>[2x]MALVDGFLELERSSGKLEWSAILQKMASDLGFSKILFGLLPKDSQDYENAFIVGNYPAAWREHYDRAGYARVDPTVSHCTQSVLPIFWEPSIYQTRKQHEFFEEASAAGLVYGL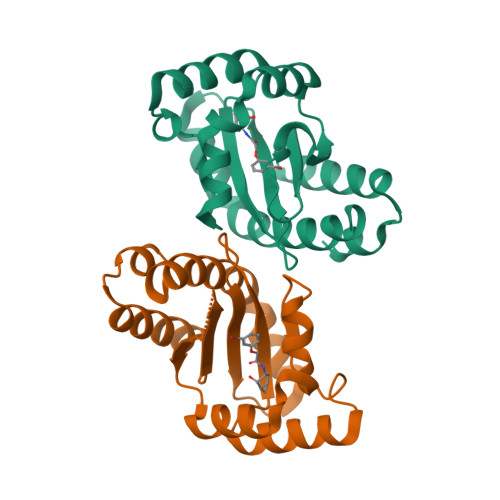TMPLHGARGELGALSLSVEAENRAEANRFMESVLPTLWMLKDYALQSGAGLAFEHPVSKPVVLTSREKEVLQWCAIGKTSWEISVICNCSEANVNFHMGNIRRKFGVTSRRVAAIMAVNLGLITL>MGHHHHHHMAGGGKHTPTPKAIIHQKFGAKASYTVEEVHDSSQSGCPGLAIPQKGPCLYRCHLQLPEFSVVSNVFKKKKDSEQSAAELALDKLGIRPQNDDLTVDEARDEIVGRIKYIFSDEFLSAEHPLGAHLRAALRRDGERCGSVPVSVIATVDAKINSRCKIINPSVESDPFLAISYVMKAAAKLADYIVASPHGLRRKNAYPSEIVEALATHVSDSLHSREVAAVYIPCIDEEVVELDTLYISSNRHYLDSIAERLGLKDGNQVMISRMFGKASCGSECRLYSEIPKKYLDNSSDASGTSNEDSSHIVKSRNARASYICGQDIHGDAILASVGYRWKSDDLDYDDVTVNSFYRICCGMSPNGIYKISRQAVIAAQLPFAFTTKSNWRGPLPREILGLFCHQHRLAEPILSSSTAPVKSLSDIFRSHKKLKVSGVDDANENLSRQKEDTPGLGHGFRCEVKIFTKSQDLVLECSPRKFYEKENDAIQNASLKALLWFSKFFADLDVDGEQSCDTDDDQDTKSSSPNVFAAPPILQKEHSSESKNTNVLSAEKRVQSITNGSVVSICYSLSLAVDPEYSSDGESPREDNESNEEMESEYSANCESSVEPIESNEEIEFEVGTGSMNPHIESEVTQMTVGEYASFKMTPPDAAEALILAVGSDTVRIRSLLSERPCLNYNILLLGVKGPSEERMEAAFFKPPLSKQRVEYALKHIRESSASTLVDFGCGSGSLLDSLLDYPTSLQTIIGVDISPKGLARAAKMLHVKLNKEACNVKSATLYDGSILEFDSRLHDVDIGTCLEVIEHMEEDQACEFGEKVLSLFHPKLLIVSTPNYE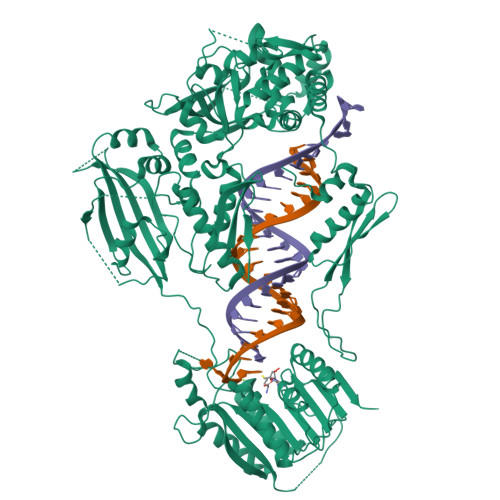FNTILQRSTPETQEENNSEPQLPKFRNHDHKFEWTREQFNQWASKLGKRHNYSVEFSGVGGSGEVEPGFASQIAIFRREASSVENVAESSMQPYKVIWEWKKEDVEKKKTDL[2x]>MDVFAKHAVSLESPAVRHYEITPSDSTDLARRPRALRVQTGGTLVLRDETGITVTYTVFAGEILPVRPVRVLATGTTATAVGWE[11x];>[29x]MPEGADPVAEVKTALAGFLKEVKGFQDDVKTRLQQQEERVTMLQTKTYAGRHALAAAATEEAPHQKAFAAYLRTGDDDGLRGLSLEGKALNSAVAAEGGYLVDPQTSETIRGVLRSTASLRQIASVVNVEATSFDVLVDKTDMGSGWASETAALSETATPQIDRITIPLHELAAMPKASQRLLDDSAFDIETWLANRIADKFARAEAAAFISGDGVDKPTGFLTKTKVANGAWAWGSLGYVATGAAGDFAAVNASDAVVDLVYALGAEYRANASFVMNSKTAGAVRKMKDADGRFLWADSLAAGEPARLMGYPVLIAEDMPDIAANAYAIAFGDFGNGYTIAERPDLRVLRDPFSAKPHVLFYASKRVGGDVSDFAAIKLLKFAAS;>[2x]MIALGLGLGLAANGGPALRRYAVNGVAPVAVLDFERHFLSHPLALTRATSATYADALRAVQTAPADTPRYDYSTGKRALLLEASATNLLPNSAQFEAASWGKTRASVLANAALAPNGTMTADKLVEDTSNNSHFVARTGTQIAAGTSVTASIFVKAAERRWFALVTADSANAFRTTYFDLQTGTLGVVSQGAAGHVAQIVAAGNGWYRCSVTQTQAASGNF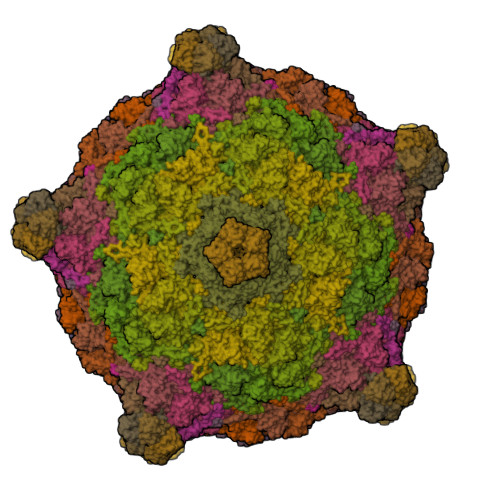NFYPSVASANGATSYPGDGASGLYLWGAQLEAGAAVSSVIPTEAAAVTRAADLASVAVAAGSYDLRRVDAAGTAVTKGVAHPGGALTIGAGSLYLLSLFPAGAL> MSHQNQLIPQAYISNFHNRLTNEDDGIPIFTMAQQTRQHKRAKVVNYAEYDNDLFDEFNMNGSNFNNADTHYKDNAVSHENTPA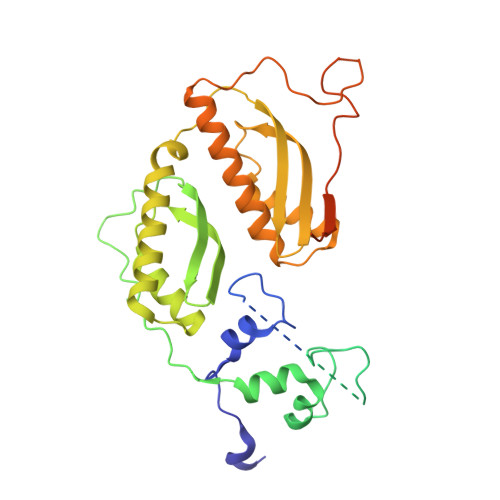LTNGVTMDGSEYNVLENMNGADSIISNNKYDAGSNMVVESLSGLNSNNNASNGPSNKAQAQDIGNAVLPDLQDQHHNPFNILRYPKIRDTFINGKVVSPYRLNTDQETKANANSGEAIMIPITLDIEHMGHTIKDQFLWNYNDDSISPEEFASIYCKDLDMTSATLQTQIANIIKEQLKDLENIAATEIMSDLHVIINLTCNLQDRFFEDNFQWNLNDKSLTPERFATSIVQDLGLTREFIPLISQSLHETILKIKKDWVDGHLIQDHVPNDAAFGYLSGIRLDIDELGSNWCPRVEILTKEEIQKREIEKERNLRRLKRETDRLSRRGRRRLDDLETTMRM> GAGCGACCTGTACGGACATC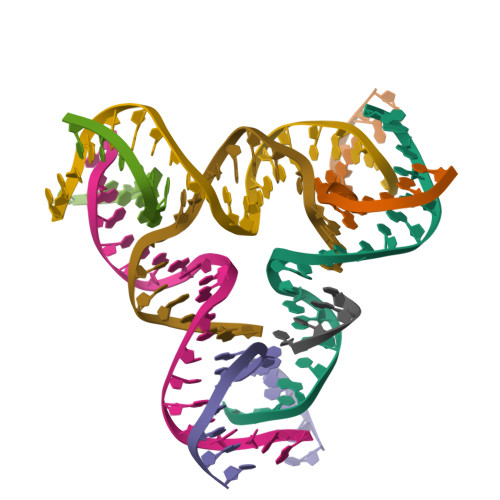A;> AACCTACCTGGCAGGACGACT;> CACGAGCCTGATCGGACAAGA;> TCTGATGTGGTAGGT;> TGTCTTGTGGTCGC;> TAGTCGTGGCTCG;> CCGT;> ACACCGATCACCTGCCA> ENFRKVRSEEAPAGCGAEGGGPGSGPFADLAPGAVHMRVKEGSKIRNLMAFATASMAQPATRAIVFSGCGRATTKTVTCAEILKRRLAGLHQVTRLRYRSVREVWQSLPPGPTQGQTPGEPAASLSVLKNVPGLAILLSKDALDPRQPGYQPPNPHPGPSSPPAAPASKRSLGEPAAGEGSAKRSQPE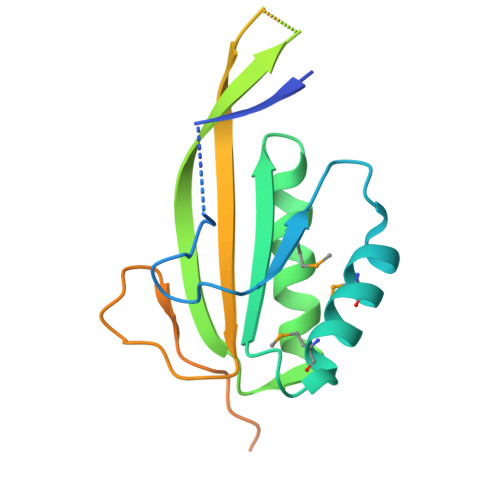PGVADEDQTA6-(4-methylphenyl)sulfanyl-2~{H}-[1,2,4]triazolo[4,3-b]pyridazin-3-one | C12 H10 N4 O S | 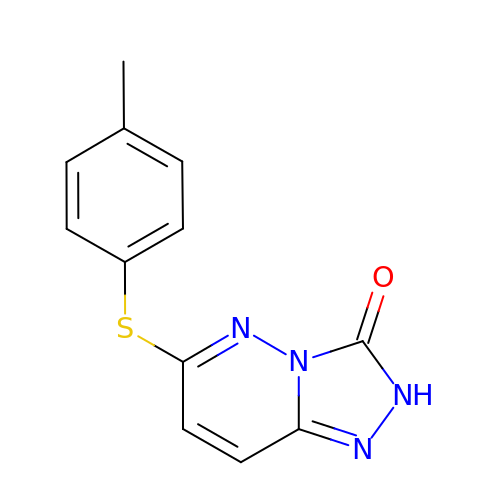SVJSYMYGSKESLF-UHFFFAOYSA-N> XNLAALRSELQALRREGFSPERLAALESRLQALERRLAALRSRLQA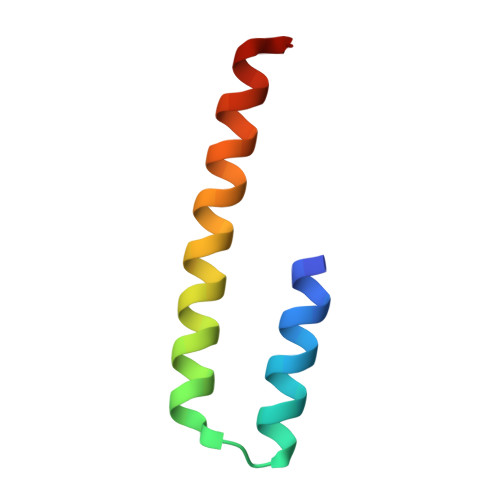LRGX> GPMATVFRQENVDDYYDTGEELGSGQFAVVKKCREKSTGLQYAAKFIKKRRTKSSRRGVSREDIER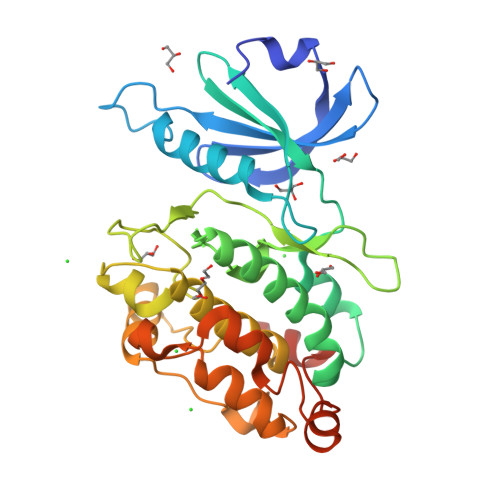EVSILKEIQHPNVITLHEVYENKTDVILILELVAGGELFDFLAEKESLTEEEATEFLKQILNGVYYLHSLQIAHFDLKPENIMLLDRNVPKPRIKIIDFGLAHKIDFGNEFKNIFGTPEFVAPEIVNYEPLGLEADMWSIGVITYILLSGASPFLGDTKQETLANVSAVNYEFEDEYFSNTSALAKDFIRRLLVKDPKKRMTIQDSLQHPWIKPKDTQQALSRKAEAVNMEKFKKFAARKKWKQAVR>[2x]MRSNLLAFSIVASLGLAQVAHAAEGMWVPQQLPEIAGPLQKAGLKLSPEQLANLTGDPMGAVVALGGCTASFVSPQGLVVTNHHCAYGAIQLNSTAQKNLIKDGFNAPTLKDELSAGPNARVFVLDQITDVTAQAKAAIAGAGNDPLARSRALDAFDKAQVAACEADAGFRCRLYSFSGGNTYRLFRNMEIKDVRLVYAPPGSVGKFGGDVDNWMWPRHTGDFSFYRAYVGKDGKPAAFAADNVPYQPKHFLKFADQPLGADDFVMVAGYPGRTNRYALAGEFNETASFTYPTIAKHYNAVLKMIADAGKADADVKVKYAATAASMNNVAKNYLGQLEGFKRIDAAGQKQAEEAAVLAWLKKQGAAGKPALAAHAQLLKHLDTSKSTRERDLFVGQFNNTSAVGAAITLYRLSIERSKPDAEREAGYQERDLTTIEGGLKQMDRRYVAKMDQQLQTYWLDQYVALPAAQRDNEVLNKWLAGSDAAAVKSLVNKLGGTELGSLDTRLKWFKADRAAFEASNDPAIQYAVAVMPALLKQEEQKKIREGESLTARPLYLQAVADYKKSQGEFVYPDANLSLRITFGNVMGYGKDGVKYTPFTTLEGVAAKETGEDPFDSPKALLDAVKAKRYGGLEDKRLGSVPVNFLSNLDITGGNSGSPVLDANGKLVGLAFDGNWESVSSNWVFDPVMTRMIAVDSRYMQWIMQEVAPAPQLLKELNLAK

Family S46 peptidases are serine proteases showing dipeptidyl peptidase activity and are widely distributed in Bacteroidetes and Proteobacteria, but are not found in mammals. The SmDPP7 enzyme forms a homodimer, with each subunit consisting of 697 residues (Ala23-Ala719) and a molecular weight of approximately 155 kDa. Each subunit contains a catalytic double β-barrel domain harbouring the Asp-His-Ser catalytic triad (top domain) and an α-helical domain that caps the active site (bottom domain). SmDPP7 hydrolyses peptides from the N-terminus of oligopeptides, cleaving the dipeptide units (NH2-P2-P1-COOH) when the second P1 residue is a hydrophobic amino acid.

For simplicity, the following description refers primarily to subunit A of the 1.86-Å-resolution structure of the Tyr-Tyr complex of SmDPP7. The bound dipeptide was found in the active site cleft of the catalytic domain and was covered by the α-helical domain. The aromatic ring of the bound Tyr(P1) has hydrophobic contacts with the side chains of Trp214 and Ile650. The hydroxy group of the bound Tyr(P1) points toward the bottom of the S1 subsite. The side chain of bound Tyr(P2) is accommodated in the S2 subsite and has aliphatic contacts with the side chains of His84, Lys206, and Phe671. The hydroxy group of Tyr(P2) forms hydrogen bonds to the carbonyl oxygens of Phe207 and Gly209, and the side chain of Arg218 via a water molecule. Thus, specific interaction between the S2 subsite and the side chain of Tyr(P2) is limited, whereas the main-chain atoms of Tyr(P2) are tightly fixed by the side chains of Asn213, Trp214, Asn328, and Asp672. In the Tyr-Tyr complex, one of the four water molecules at the bottom of the S2 subsite in the Val-Tyr complex is replaced by the hydroxy group of Tyr(P2) and the side chain of Lys206 is well ordered due to aliphatic contacts with the side chain of Tyr(P2). Although the structure of the Tyr-Tyr complex showed hydrogen bonds to the carbonyl oxygens of Phe207 and Gly209 and the side chain of Arg218 via a water molecule, the enthalpic ﻿contribution showed little difference as compared with Phe-Tyr binding. This suggested that these hydrogen bonds do not significantly contribute to Tyr(P2) binding.> MGKEKSHINVVVIGHVDSGKSTTTGHLIYKCGGIDKRTIEKFEKEAAELGKGSFKYAWVLDKLKAERERGITIDIALWKFETPKYQVTVIDAPGHRDFIKNMITGTSQADCAILIIAGGVGEFEAGISKDGQTREHALLAFTLGVRQLIVAVNKMDSVKWDESRFQEIVKETSNFIKKVGYNPKTVPFVPISGWNGDNMIEATTNAPWYKGWEKETKAGVVKGKTLLEAIDAIEQPSRPTDKPLRLPLQDVYKIGGIGTVPVGRVETGVIKPGMVVTFAPAGVTTEVKSVEMHHEQLEQGVPGDNVGFNVKNVSVKEIRRGNVCGDAKNDPPKGCASFNATVIVLNHPG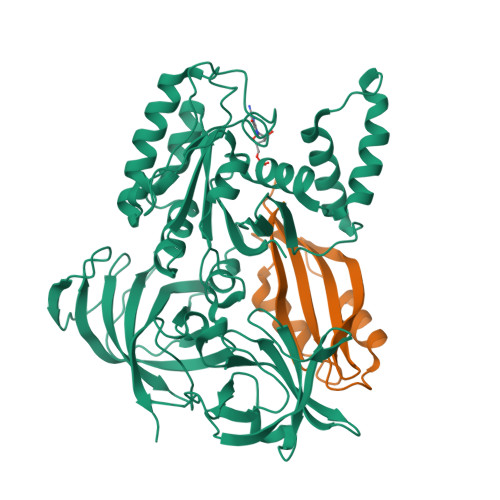QISAGYSPVLDCHTAHIACRFDELLEKNDRRSGKKLEDHPKFLKSGDAALVKFVPSKPMCVEAFSEYPPLGRFAVRDMRQTVAVGVIKSVDKTEKAAKVTKAAQKAAKK;> KPAKPAAKSIVTLDVKPWDDETNLEEMVANVKAIEMEGLTWGAHQFIPIGFGIKKLQINCVVEDDKVSLDDLQQSIEEDEDHVQSTDIAAMQKL> MEHVAFGSEDIENTLAKMDDGQLDGLAFGAIQLDGDGNILQYNAAEGDIT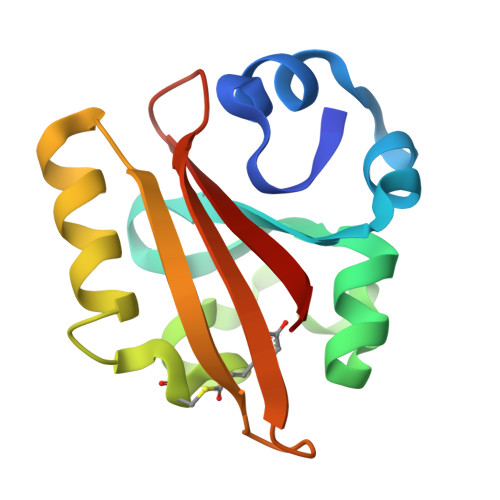SRDPKQVIGKNFFKDVAPCTDSPEFYGKFKEGVASGNLNTMFEYTFDYQMTPTKVKVHMKKALSGDSYWVFVKRV>GAMAVIDNSTKTLEQQTAQTNVAALPAITVKAEQDDTYAGGQVATSSNVGFLGSKKFLDTPFNTISYTDKYIEDKQAKDITEVIAATDPSIYTNGASGGWSENYYIRGYASSTNDMSMNGLFGITPFYRTSPEMFGRVEVLKGPSALLNGMPPAGSVGGTVNLVTKYAADEPFARLTTTYMSDAQFGGHVDVGRRFGENKEFGVRINGMYRDGDAAVNDQSKESRLFSLGLDWQGENARVFVDAYDALDHVDGVTRGVNVSTAVGIPKPPKADTLLSPDWGSVETKDKGAMIRGEYDFSDQLMAYAAYGQSTTEYKYNGASAGTITSSTGTLSSTLGQLAFDVDKKSADAGFKGKFETGSVKHQWVANATYYNHTQDDYGYRIIPGFSDPVITNIYDPNPNWGPKPEFTPPFLFHSTLSTSSFGLADTLSFAQDKVQLTLGLRHQTVKATSSVNTLPENAKSATTPGVALLIKATDKISVYANYIEGLTKGDQAPATASNPGEIFPPQKTKQQELGLKVDLGTFAHTLSAFEITKPSSYLDPSKLVNNLPTFVSDGEQRNRGIEWSFFGSPIEHVRLMGGFTYLDPELTKTKSGGNDGHTAVAVPKNQAKLGAEWDTQVAQGTLTLSGNINAVSKQYINAENTLSVPGRTLLDVGARYSTKVEDHPVTFRANIYNLTNKAYWAQPQLTNLALGAPRTYMLSVSYDF[3x]

The A. baumannii outer-membrane transporter protein, BauA, that recognises this siderophore has itself been identified as a vaccine candidate. The siderophore is known to be bound from the medium by the integral outer-membrane BauA protein. BauA has the typical outer-membrane TonB-dependent transporter (TBDT) fold with a β-barrel formed by 22 antiparallel strands, several extracellular loops, and a plug domain folded inside of the barrel. Acinetobactin is synthesized as a precursor, preacinetobactin, which rearranges non-enzymatically and irreversibly at pH >7 to give acinetobactin.

We incubated separate native protein crystals with preacinetobactin and acinetobactin compounds (both compounds preloaded with Fe3+); surprisingly in both cases, we obtained the same structure: BauA bound to a heterocomplex Fe3+-preacinetobactin-acinetobactin (1:1:1). The coordination of the iron is octahedral with four coordination atoms from preacinetobactin (one hydroxy group of the catecholate, the hydroxy of the hydroxamate, the nitrogen of the methyl oxazoline and one nitrogen (N1) of the imidazole group) and two hydroxyls from acinetobactin (the catecholate). The binding site is located inside the β-barrel similar to other siderophore complexes. BauA recognises the preacinetobactin through two direct hydrogen bonds between the hydroxamate group and Tyr312 of β7 and Arg253 of L3 and one interaction through a bridging water molecule between Asp375 and the nitrogen N2 of the imidazole, respectively. The binding site is predominantly hydrophobic in character with van der Waals interactions involving residues Trp97, Tyr125, Tyr314, Tyr378, Gly334, Gln335, Leu336, Arg379 and Leu684. Although there are no hydrogen bonds between the siderophores and the plug domain, two residues of the plug domain (Trp97 and Tyr125) do make van der Waals interactions with preacinetobactin. The acinetobactin molecule makes only one hydrogen bond (Arg253) and one van der Waals interaction (Leu684). There are no changes in the TonB region as a result of ligand binding. In the crystal structure, preacinetobactin fits into a complementary pocket; a simple molecular model shows that the same site would not bind acinetobactin due to extensive van der Waals clashes with Tyr312. The acinetobactin molecule is not itself recognised by the protein, rather it is the favorable coordination of the catechol group to the remaining two sites of Fe3+ that drives complex formation.> AEGQTNADDTLVVEASTPSLYAPQQSADPKFSRPVADTTRTMTVISEQVIKDQGATNLTDALKNVPGVGAFFAGENGNSTTGDAIYMRGADTSNSIYIDGIRDIGSVSRDTFNTEQVEVIKGPSGTDYGRSAPTGSINMISKQPRNDSGIDASASIGSAWFRRGTLDVNQVIGDTTAVRLNVMGEKTHDAGRDKVKNERYGVAPSVAFGLGTANRLYLNYLHVTQHNTPDGGIPTIGLPGYSAPSAGTAALNHSGKVDTHNFYGTDSDYDDSTTDTATMRFEHDINDNTTIRNTTRWSRVKQDYLMTAIMGGASNITQPTSDVNSWTWSRTANTKDVSNKILTNQTNLTSTFYTGSIGHDVSTGVEFTRETQTNYGVNPVTLPAVNIYHPDSSIHPGGLTRNGANANGQTDTFAIYAFDTLQITRDFELNGGIRLDNYHTEYDSATACGGSGRGAITCPTGVAKGSPVTTVDTAKSGNLMNWKAGALYHLTENGNVYINYAVSQQPPGGNNFALAQSGSGNSANRTDFKPQKANTSEIGTKWQVLDKRLLLTAALFRTDIENEVEQNDDGTYSQYGKKRVEGYEISVAGNITPAWQVIGGYTQQKATIKNGKDVAQDGSSSLPYTPEHAFTLWSQYQATDDISVGAGARYIGSMHKGSDGAVGTPAFTEGYWVADAKLGYRVNRNLDFQLNVYNLFDTDYVASINKSGYRYHPGEPRTFLLTANMHF

The ferric iron uptake (Fiu) transporter is a TBDT responsible for import of molecules containing the catecholate functional group. Members of the TonB-dependent transporter (TBDT)3 family drive transport of their substrates through interaction with the energy-transducing protein TonB. The structure of Fiu consists of a 22-stranded transmembrane β-barrel characteristic of the TBDT superfamily, with a number of extended extracellular loops that might serve in the initial steps of substrate binding. In addition to its role in iron uptake, Fiu has also been shown to be important for sensitivity to antimicrobials that share the common feature of a catecholate functional group or the analogous dihydroxypyridine moiety.

The structure of Fiu was solved in three different crystal forms, revealing Fiu in two distinct states. In crystal state 1, extracellular loops 7–9 of the β-barrel were disordered, as was the extended extracellular loop of the N-terminal plug domain, which occluded the lumen of the Fiu β-barrel. The disorder of the plug domain loop in crystal state 1 opens a large cavity in the interior of Fiu to the external environment, whereas, in crystal state 2, this cavity is present but occluded in the lumen of the Fiu barrel. In crystal state 1, removal of this subdomain opens a large channel between the periplasm and the external environment. Therefore, it is likely to be undesirable for Fiu to exist in the open-channel state, which would result from simultaneous displacement of the plug subdomain and disorder of the plug domain loop. Although the internal cavity would be inaccessible to Fe–DHB in the closed state, because of the fully ordered plug loop, it would be accessible in state 1, as this loop is disordered. Glu-108 is disordered in the open state of Fiu and is not within bonding distance of docked Fe–DHB (5.3 Å) but may form interactions with polar substrate groups in vivo or generally stabilize the binding pocket. The observed crystal states may represent conformational transitions the receptor undergoes during substrate binding and transport.>SNVPHKSSLPEGI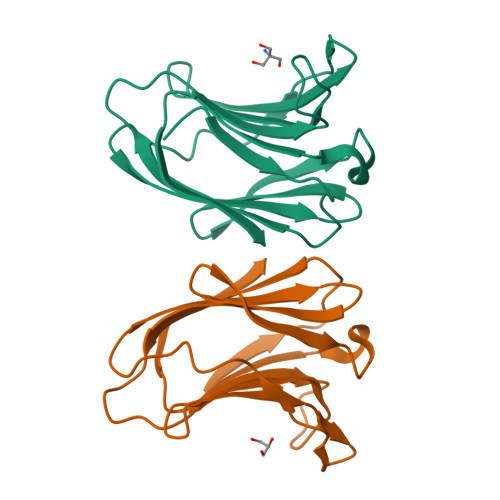RPSTVLRIRGLVPPNASRFHVNLLCGEEQGSDAALHFNPRLDTSEVVFNSKEQGSWGREERGPGVPFQRGQPFEVLIIASDDGFKAVVGDAQYHHFRHRLPLARVRLVEVGGDVQLDSVRIF[2x]> SGWCDPRWYDPFMC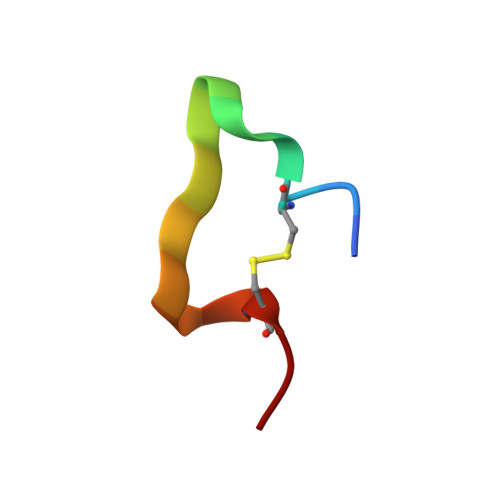EH> GSRIKQNPETTFEVYVEVAYPRTGGTLSDPEVQRQFPEDYSDQEVLQTLTKFCFPFYVDSLTVSQVGQNFTFVLTDID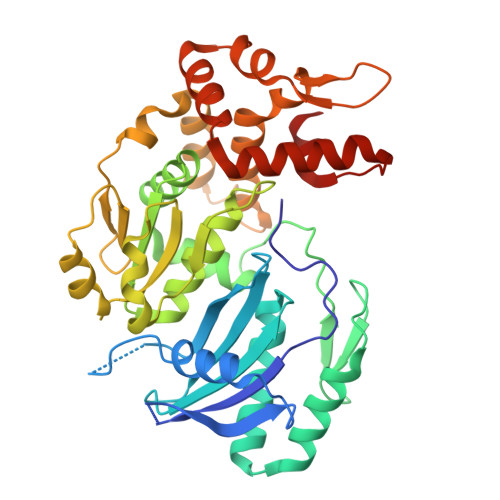SKQRFGFCRLSSGAKSCFCILSYLPWFEVFYKLLNILADYTTKRQENQWNELLETLHKLPIPDPGVSVHLSVHSYFTVPDTRELPSIPENRNLTEYFVAVDVNNMLHLYASMLYERRILIICSKLSTLTACIHGSAAMLYPMYWQHVYIPVLPPHLLDYCCAPMPYLIGIHLSLMEKVRNMALDDVVILNVDTNTLETPFDDLQSLPNDVISSLKNRLKKVSTTTGDGVARAFLKAQAAFFGSYRNALKIEPEEPITFCEEAFVSHYRSGAMRQFLQNATQLQLFKQFIDGRLDLLNSGEGFSDVFEEEINMGEY> MALMTWTAAEFGTNVGFADDQHKTIFDMVNKLHDTAATGNRSEIGKQL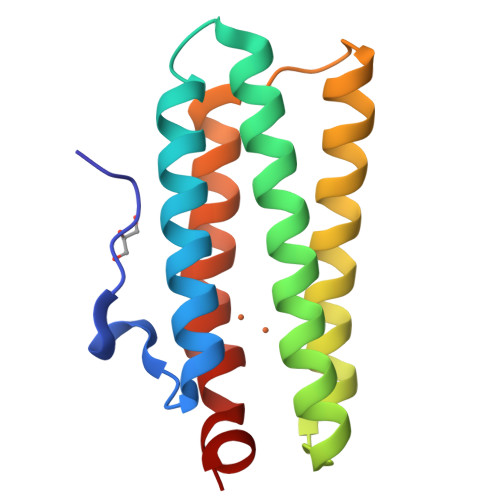DALIDYVVMHFKSEETEMQKKGYADFAAHKAEHDKLVGVCADLQKKFHAGEAEVNQDTTRFVRDWYVNHIPKVDKLYGPCLSA> MASSHHHHHHSSGLVPRGSTEATAGTVTVNAITSDDVINASEAAG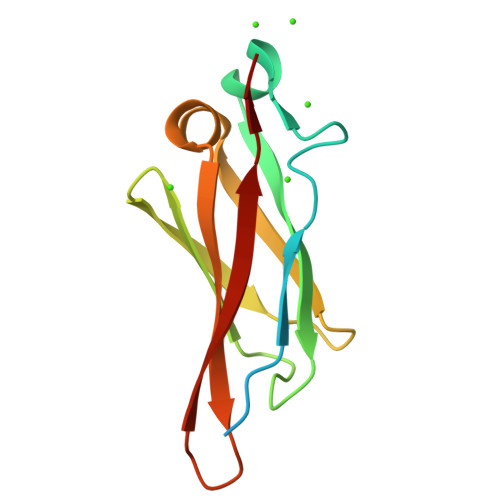TVAVSGTATGGDIAEGDTVTLEINGETYTTTVDANGEWSVDVAGSDLAADTAFDAVVTSSDAAGNTVDTTGSSTHTVD> MGSSHHHHHHSQDPDQPGNSSLENLPPVAASIEQLLERQWSEGQQFLLEQGTPSDILGMLKSLHQLQVENRRLEEQIKNLTAKKERLQLLNAQLSVPF;> MHSPNPLLVAPTPPALQK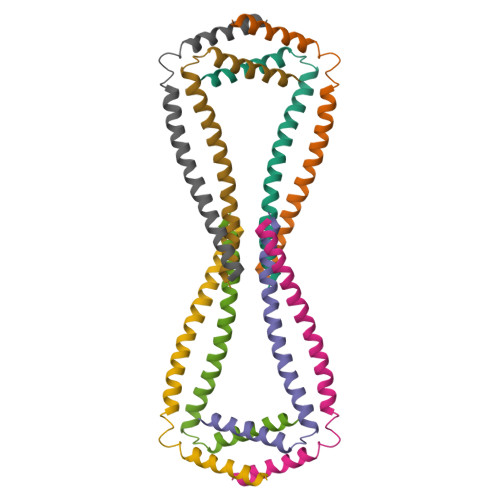LLESFKIQYLQFLAYTKTPQYKASLQELLGQEKEKNAQLLGAAQQLLSHCQAQKEEIRRLFQQK>STITRPIIELSNTCDKIAEGNLEAEVPHQNRADEIGILAKSIERLRRSLKVA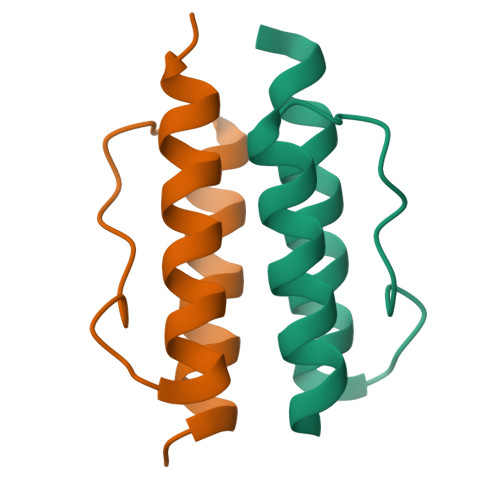ME[4x]>NLQQFKNMIQCAGTRTWTAYINYGCYCGKGGSGTPVDKLDRCCYTHDHCYNQADSIPGCNPNIKTYSYTCTQPNITCTRTADACAKFLCDCDRTAAICFASAPYNINNI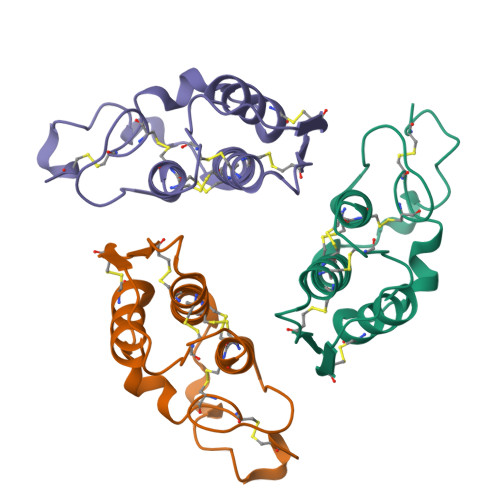MISASNSCQ[3x]(4S)-5-carbamimidamido-4-hydroxy-2-oxopentanoic acid | C6 H11 N3 O4 | 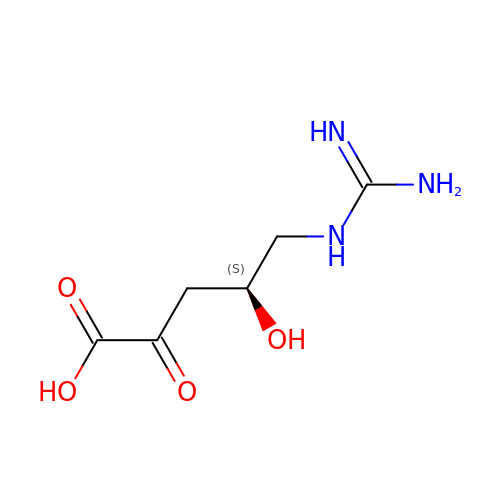RPBOKETVUMOUHD-VKHMYHEASA-N3,8-dimethoxy-1-oxidanyl-anthracene-9,10-dione 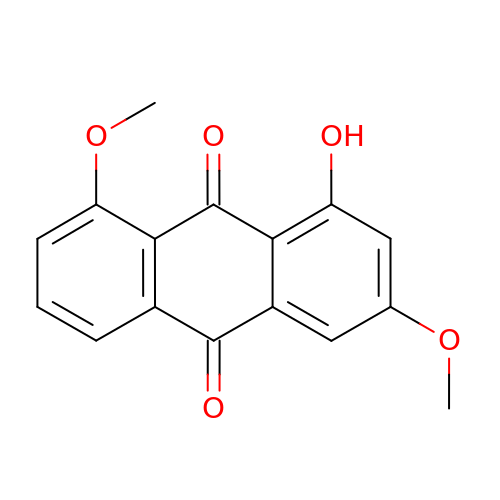| C16 H12 O5 | GAFPZYFLMZLWCQ-UHFFFAOYSA-N>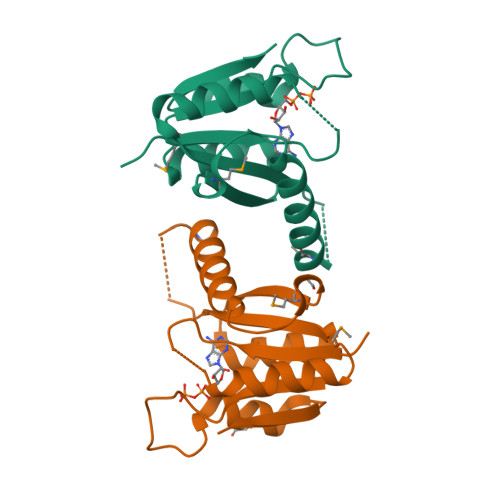SNAMILVPIDISDKEFTERIISHVESEARIDDAEVHFLTVIPSLPYYASLGMAYTAELPGMDELREGSETQLKEIAKKFSIPEDRMHFHVAEGSPKDKILALAKSLPADLVIIASHRPDITTYLLGSNAAAVVRHAECSVLVVR[2x]>[4x]GGGSMEVVGDFEYSKRDLVGHGAFAVVFRGRHRQKTDWEVAIKSINKKNLSKSQILLGKEIKILKELQHENIVALYDVQELPNSVFLVMEYCNGGDLADYL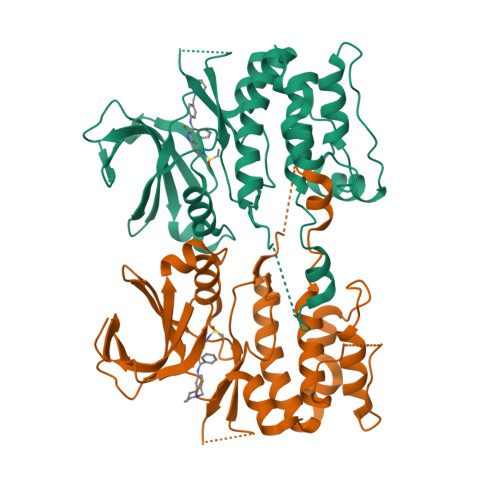QAKGTLSEDTIRVFLHQIAAAMRILHSKGIIHRDLKPQNILLSYANRRKSSVSGIRIKIADFGFARYLHSNMMAADLCGSPMYMAPEVIMSQHYDAKADLWSIGTVIYQCLVGKPPFQANSPQDLRMFYEKNRSLMPSIPRETSPYLANLLLGLLQRNQKDRMDFEAFFSHPFLEQGPV> NEVTLLDSRSVQGELGWIASPLEGGWEEVSIMDEKNTPIRTYQVCNVMEPSQNNWLRTDWITREGAQRVYIEIKFTLRDCNSLPGVMGTCKETFNLYYYESDNDKERFIRENQFVKIDTIAADESFTQVDIGDRIMKLNTEIRDVGPLSKKGFYLAFQDVGACIALVSVRVFYKK;> SIVLEPIYWNSSNSKFLPGQGLVLYPQIGDKLDIICPKVDSKTVGQYEYYKVYMVDKDQADRCTIKKENTPLLNCAKPDQDIKFTIKFQEFSPNLWGLEFQKNKDYYIISTS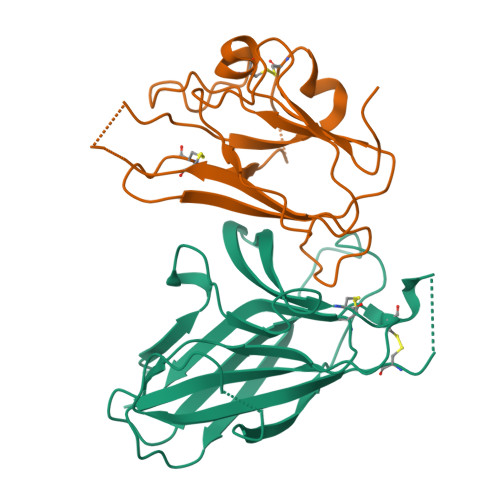NGSLEGLDNQEGGVCQTRAMKILMKVGQDAS> GDITHMEKLGDIC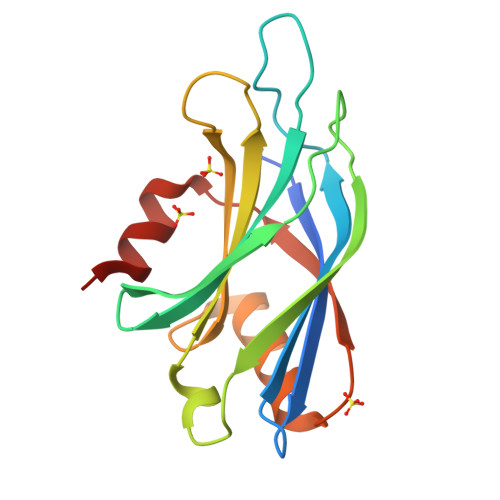FSLRYVPTAGKLTVVILEAKNLKKMDVGGLSDPYVKIHLMQNGKRLKKKKTTIKKNTLNPYYNESFSFEVPFEQIQKVQVVVTVLDYDKIGKNDAIGKVFVGYNSTGAELRHWSDMLANPRRPIAQWHTLQVEEEVDAMLAVKK~{N}-[(3~{R})-2-oxidanylideneazepan-3-yl]furan-2-carboxamide 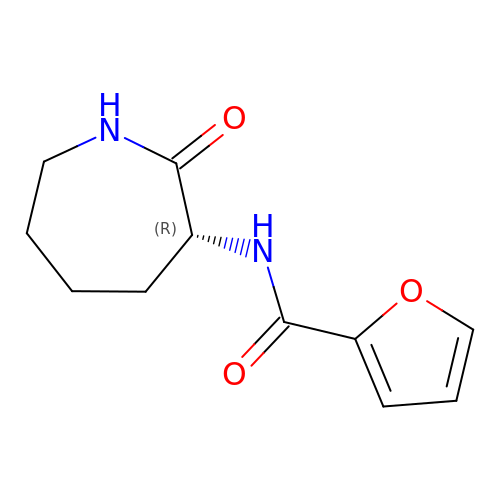| C11 H14 N2 O3 | KMCPPIBDTMYPRI-MRVPVSSYSA-N(1~{S},5~{S},6~{R})-10-(1,3-benzothiazol-6-ylsulfonyl)-5-(methoxymethyl)-3-(pyridin-2-ylmethyl)-3,10-diazabicyclo[4.3.1]decan-2-one | C23 H26 N4 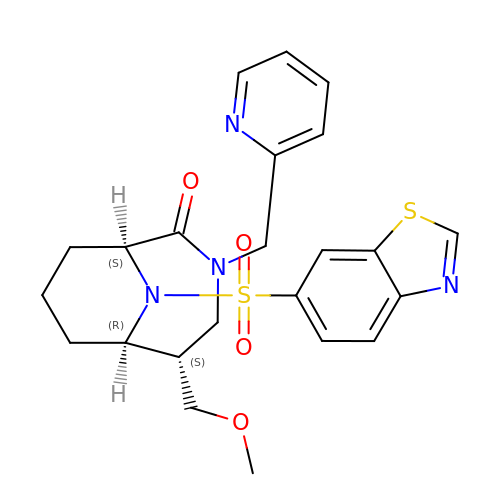O4 S2 | CVICEWHMKVUYQU-HBGVWJBISA-N> MHHHHHHMLEAKFEEASLFKRIIDGFKDCVQLVNFQCKEDGIIAQAVDDSRVLLVSLEIGVEAFQEYACAHPVTLGMDLTSLSKILRCGNNTDTLTLIADNTPDSIILLFEDTKKDRIAEYSLKLMDIDADFLKIEELQYDSTLSLPSSEFSKIVRDLSQLSDSINIMITKETIKFVADGDIGSGSVIIKPFVDMEHPETSIKLEMDQPVDLTFGAKYLLDIIKGSSLSDRVGIRLSSEAPALFQFDLKSGFLQFFLAPKFNDEE

PCNA is a ring-shaped homotrimeric protein, with each subunit consisting of two domains connected by a flexible linker called the inter-domain connecting loop (IDCL). CAF-1 association with replicating DNA, and the targeting of newly synthesized histones to sites of DNA replication and repair requires its interaction with proliferating cell nuclear antigen (PCNA), the eukaryotic sliding clamp that acts as a processivity factor for polymerases during DNA synthesis. Recruitment of PCNA-interacting proteins to replication forks is generally mediated by a conserved sequence in these proteins called a PCNA-interacting protein (PIP) motif that interacts with PCNA in a region between the two domains on a single subunit near the IDCL. In this study, we focused on three separation-of-function amino acid substitutions in PCNA that cause defective gene silencing and exhibit reduced CAF-1 association with chromatin in vivo, as well as inhibit binding to CAF-1 in vitro partially or completely (D41A/D42A, R61A/D63A, and L126A/I128A).

The X-ray crystal structure of the R61A/D63A mutant protein was determined to a resolution of 3.3 Å. The R61A substitution is located in β strand E1 and the D63A substitution is located in loop F (residues 62–65) in domain 1 of PCNA. The R61A/D63A substitutions are located on the side of PCNA adjacent to and within loop F (residues 62 to 65), which is over 30 Å away from the PIP-interacting region. At the site of the substitutions, there are small backbone changes around residues 61 and 62. Although the substitutions at residues 61 and 63 only appear to cause minor structural changes near these positions, they produce significant changes in loop B (residues 21 to 24), a region of the PCNA monomer that is more than 30 Å away from the substitutions. Compared to the wild-type structure, there are significant backbone changes in the structure of the R61A/D63D mutant PCNA protein in loop B. The α carbon of residue 21 has moved by 1.2 Å relative to its position in the wild-type PCNA structure, and the α carbon of residue 22 has moved by 2.6 Å. Although the precise reason for this induced, long-range structural change is unclear, it is likely mediated through β strand A1 (residues 2 to 6) and α helix A1 (residues 9 to 20). The overall shape of this cavity is similarly altered in the R61A/D63A mutant protein structure. Here, there are alterations (>1 Å) in the backbone of several amino acid residues along the edges of the cavity, including residues 21 and 22 in loop B and residues 123 and 124 in the IDCL. While the D41A/D42A and L126A/I128A mutant proteins are completely defective in CAF-1 binding, the R61A/D63A mutant is only partially defective in CAF-1 binding.>ACYCRIPACIAGERRAGTCAYQGRAWAACC[4x]

Defensins are a family of antimicrobial peptides of innate immunity broadly active against bacteria, viruses and toxins. They are small (2–5 kDa), stabilized structurally by three disulfide bonds, form oligomers, and are divided into α, β and θ structural classes. The canonical dimer interface of HNP1 is formed by the antiparallel extensions of the β2 strands stabilized by the reciprocal main-chain hydrogen bonds contributed by Thr18 and Ile20, and the hydrophobic packing of the side chains of Tyr16, Tyr21, Trp26, Phe28 and the Cys2–Cys30 and Cys4–Cys19 disulfides. Further analysis of probable quaternary structures by the Protein Interfaces, Surfaces and Assemblies (PISA) software indicates that the HNP1 dimer forms a tetramer or dimer of dimers in a crystal.

Y16A/I20A/L25A/F28A-HNP1 forms a dimer which is very similar to the Y16A/F28A-HNP1 dimer (the average RMSDs between 60 equivalent Cα-atoms of 0.4 Å). Solvent-accessible surface buried due to Y16A/I20A/L25A/F28A-HNP1 and Y16A/F28A-HNP1 dimer formation corresponds to 490 and 495 Å2 per monomer, respectively, indicating that these dimers are energetically indistinguishable. Surprisingly, although Y16A/I20A/L25A/F28A-HNP1 has mutated Ile20 and Leu25 that were previously identified as essential for wild type tetramer formation, analysis of intermolecular contacts within the crystal indicates that Y16A/I20A/L25A/F28A-HNP1 dimers arrange into a tetramer resembling closely the wild-type tetramer architecture. Replacement of Ile20 and Leu25 side chains at the tetramer interface by less ‘bulky’ side chains of Ala allows Y16A/I20A/L25A/F28A-HNP1 dimers to pack more tightly together. The buried interface area for Y16A/I20A/L25A/F28A-HNP1 tetramer formation is 1450 Å2 per dimer as compared to 1140 Å2 buried at the wild type HNP1 tetramer interface. In addition, the canonical dimer formed by the quadruple mutant displayed a larger interface than wild-type. HNP1 bound to immobilized HNP1 with a 20-fold greater response at 8000 nM than Y16A/I20A/L25A/F28A-HNP1 bound to HNP1, and HNP1 bound to immobilized gp120 with an 8-fold greater response at 8000 nM than Y16A/I20A/L25A/F28A-HNP1 bound to gp120. All HNP1 analogs except Y16A/I20A/L25A/F28A-HNP1 bound N36 in a dose-dependent fashion, reflected by increasing fluorescence polarization values with the increase in defensin concentration. However, the inhibitory activity of Y16A/F28A and Y16A/I20A/L25A/F28A in particular was greatly suppressed with the latter yielding an IC50 95-fold higher than that of wild type HNP1. Notably, Y16A/I20A/L25A/F28A-HNP1 barely showed any activity at the maximum tested concentration of 256 µg/mL against S. aureus, whereas its activity remained less than vLD99.9 against E. coli and its vLD99.9 against B. cereus was 11-fold higher than HNP1.> SLEA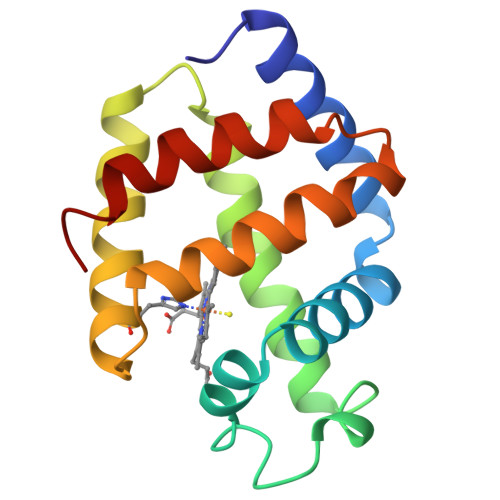AQKSNVTSSWAKASAAWGTAGPEFFMALFDAHDDVFAKFSGLFSGAAKGTVKNTPEMAAQAQSFKGLVSNWVDNLDNAGALEGQCKTFAANHKARGISAGQLEAAFKVLSGFMKSYGGDEGAWTAVAGALMGEIEPDM(2~{R},3~{R},4~{S},5~{R})-2-[6-azanyl-8-[3-[[(2~{R},3~{S},4~{R},5~{R})-5-[6-(2-azanylethylamino)purin-9-yl]-3,4-bis(oxidanyl)oxolan-2-yl]methoxy]prop-1-ynyl]purin-9-yl]-5-(hydroxymethyl)oxolane-3,4-diol 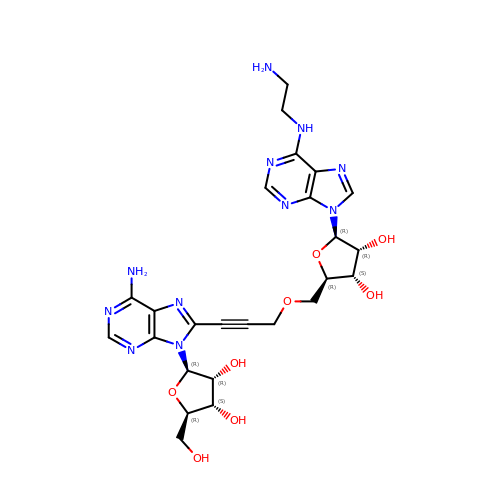| C25 H31 N11 O8 | SCMIFBNZCXBOAA-AKONZDDMSA-N> LCEEGLKRLQQMLAEYQAQSDVPQEVCDQILEAAKESSVGEDGVRSQVKIRKPNGKNNIRYEYDLDHIDCKKNEITFYRHINYSDGSKRKIQYTVGIEGFVDIYDFVNVQKCDAQVYDTKTSKTVGGRKIINSEFAGKTVTTKGGDVRFDSDGFPDFTPYSKKTVRVIGLTGDMANDVPLAMARAKITKYDKSKYVWHHHQDGKTM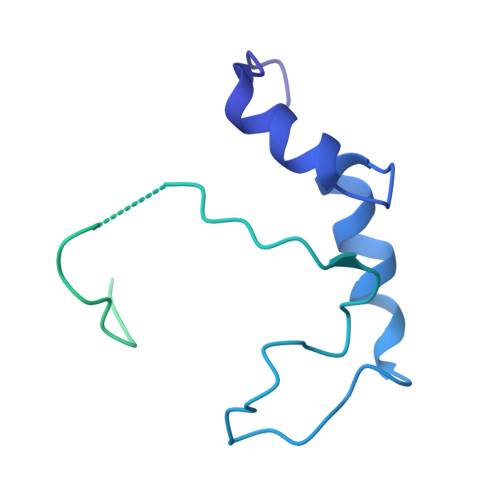MLIPKSVHSVRNGGVAATGGRSVIQHNLLNPNNKLNYSSPEELV>EDRPSKAPSFWYKIDPSHTQGYRTVQLVWKTLPPFEANGKILDYEVTLTRWKSHLQNYTVNATKLTVNLTNDRYLATLTVRNLVGKSDAAVLTIPACDFQATHPVMDLKAFPKDNMLWVEWTTPRESVKKYILEWCVLSDKAPCITDWQQEDGTVHRTYLRGNLAESKCYLITVTPVYADGPGSPESIKAYLKQAPPSKGPTVRTKKVGKNEAVLEWDQLPVDVQNGFIRNYTIFYRTIIGNETAVNVDSSHTEYTLS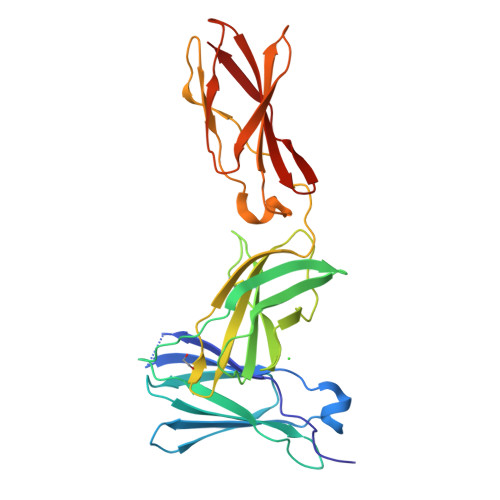SLTSDTLYMVRMAAYTDEGGKDGPEFTFTT[2x]> SMQDPTIFEERHLKYISQLGKGNFGSVELCRYDPLGDNTGALVAVKQLQHSGPDQQRDFQREIQILKALHSDFIVKYRGVSYGPGRQSLRLVMEYLPSGCLRDFLQRHRARLDASRLLLYSSQICKGMEYLGSRRCVHRALAARNILVESEAHVKIADFGLAKLLPLDKDYYVVREPGQSPIFWYAPESLSDNIFSRQSDVWSFGVVLYELFTYCDKSCSPSAEFLRMMGSERDVPALSRLLELLEEGQRLPAPPACPAEVHELMKLCWAPSPQDRPSFSALGPQLDMLWSGSR

Janus kinases (JAKs) are a family of cytoplasmatic tyrosine kinases that are attractive targets for the development of anti-inflammatory drugs given their roles in cytokine signaling. While the other isoforms of the Janus kinase family (JAK1, JAK2, and TYK2) have a broad spectrum of functions in different tissues, JAK3 plays a specific role in the development of immune-competent cells (Ghoreschi et al., 2009). In our quest for a highly selective JAK3 probe, we aimed to exploit a non-catalytic cysteine (C909), which is not present in the other JAK family members. C909 is situated in the solvent-exposed front part of the ATP binding site, where the other isoforms possess a serine residue (Chrencik et al., 2010).

High resolution crystal structures of 4 and 5 in complex with JAK3 were determined. Both compounds showed the expected orientation of the hinge binding motif featuring the typical bidentate hydrogen bonding pattern. While the complex of JAK3 with 4 only revealed the non-covalent binding mode, the structure in complex with 5 displayed the coexistence of the non-covalently and the covalently bound inhibitor 5. Furthermore, we observed a yet unprecedented binding pocket formed by R911, D912, and R953. This unique feature is induced by interactions of the nitrile moieties of 4 and 5 with R911, thereby generating a distinct cavity in the protein surface. Structural comparison with other JAK3 structures reveals that the side chain of R911 is dramatically reoriented and forms a hydrogen bond with the inhibitors nitrile and nitrogen. The guanidine moiety of R953 is flipped approximately 180° toward the nitrile group of 4 and thereby forms the ceiling of this arginine pocket. Alignment of the other 16 available JAK3 crystal structures revealed that the orientation of the aforementioned arginine residues is conserved in those structures, confirming the induction of the arginine pocket to be a unique feature of our inhibitor class. While 4 rapidly diffuses from JAK1, JAK2, and TYK2 with residence times below 1.4 min (lower detection limit), a prolonged residence time of 50 min on JAK3 was observed. BRET experiments using the JAK3 mutant R953A, as well as the double mutant R911A/R953A, showed similar affinity of 4, suggesting that the induction of the arginine cavity did not significantly affect inhibitor potency.>MGSLTEDGLSYKEKFVVRSYEVGSNKTATVETIANLLQEVGCNHAQSV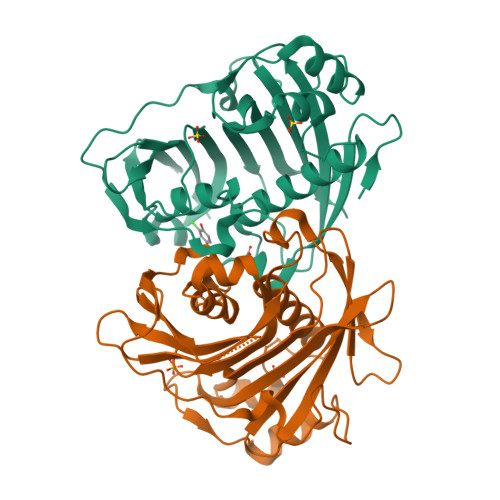GFSTDGFATTTTMRKLHLIWVTARMHIEIYKYPAWGDVVEIETWCQSEGRIGTRRDWILKDSVTGEVTGRATSKWVMMNQDTRRLQKVSDDVRDEYLVFCPQEPRLAFPEENNRSLKKIPKLEDPAQYSMIGLKPRRADLDMNQHVNNVTYIGWVLESIPQEIVDTHELQVITLDYRRECQQDDVVDSLTTTTSEIGGTNGSATSGTQGHNDSQFLHLLRLSGDGQEINRGTTLWRKKPSSHHHHHH[2x]>SMEHRYLGNSGFKVPALGFGTGTFGGQGPLFSAWGNTDVAGARRIIDICLDAGVNLFDTADVYSNGASESILGAALKGRRDKAIVSTKLSLRIGEGPNDVGSSRHHLIAATNAALQRLDTDYIDILQLHAFDAMTPVEQVLGTLDDLVRAGKVRYIGLSNFSGWQLMKSLAAADRLGLQRYVANQTYYSLIGRDYEWELMPLGIDQGVGAIVWSPLGWGRLTGKIRRGQPLPAGSRLHDTAGFAPPVDDERLYRVVDAMDEVALETGKTLPQIALNWLLQRPTVASVLIGARDEEQLMQNLGALGWQLTTEQVARLDAASAVTPPYPYYPYWNGQFAER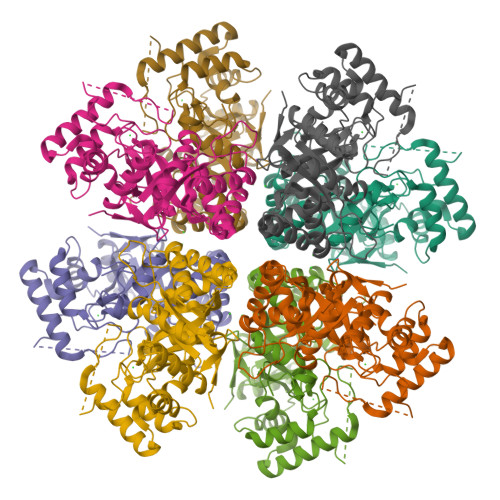SPVAV[3x]> GATGRTTIAIDPVTRIEGHLKAEVVVENGKVVDARLSGGMYRGFETILRGRDPRDASQIVQRICGVCPTAHSTASVLALDEAFGAKVPNNGRITRNLIFGANYLQSHILHFYHLSAQDFVQGPDTAPFVPRFPKSDLRLSKELNKAGVDQYIEALEVRRICHEMVALFGGRMPHVQGQVVGGATEIPTKEKLVEYAARFKKVRDFVEQKYVPVVYTIGSKYKDMFKVGQGFKAALCVGAFPLDNSGKKHLFMPGVYAKGKDMPFDPSKIKEYVKYSWFAEETTGLNYKEGKTIPAPDKAG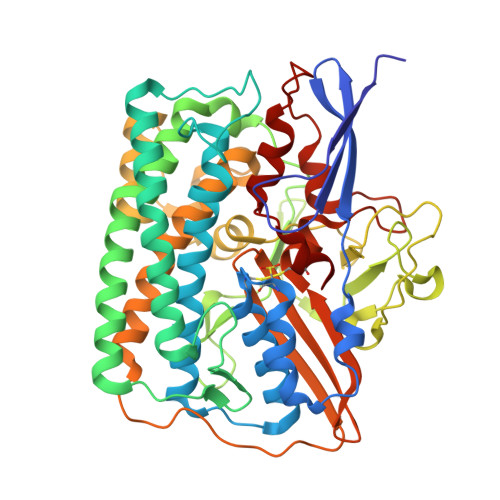AYSFVKAPRYDGLSLEVGPLARMWVNNPELSPVGKKLLKDLFGISAKKFRDLGEEAAFSLMGRHVARAEETYYMLGAIEGWLKEIKAGEDTVVMPAVPASAEGTGFTEAPRGSLLHYVKVKDSKIDNYQIVSASLWNCNPRDDMGQRGAVEEALIGIPVDDIQNPVNVARLIRAFDPULGCAVH> MSEEILFDCLHAEIVNYCLDSNKEHDLATLEYIGFTTGYRLIERLTRE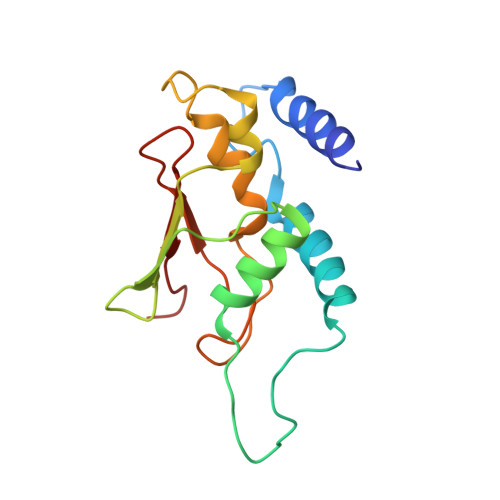VSRFKDELETMKFICTDFWMLIYKKQVDNLRTNNHGMYVVQDKAFRFLTRISPGTKQLEHAPKFVAFTCGLVRGALSNLGINSTVTAEVQSIPACKFHIEVNRN Diacylglycerol (DAG) is a versatile lipid whose 1,2-sn-stereoisomer serves both as second messenger in signal transduction pathways that control vital cellular processes, and as metabolic precursor for downstream signaling lipids such as phosphatidic acid. Effector proteins translocate to available DAG pools in the membranes by using conserved homology 1 (C1) domains as DAG-sensing modules. PKCs define a central DAG-sensing node in intracellular phosphoinositide signaling pathways that regulate cell growth, differentiation, apoptosis, and motility. Herein, we report the high-resolution crystal structures of a C1 domain (C1B from PKCδ) complexed to DAG and to each of four potent PKC agonists that produce different biological readouts and that command intense therapeutic interest.

We crystallized apo C1Bδ under conditions similar to those used for the C1Bδ-DAG complex (but without detergent) for a direct comparison. We found the structure to be identical to the previously reported apo structure (1PTQ17) with a backbone r.m.s.d. of 0.4 Å. The apo structure superimposes well onto the structures of DAG-complexed C1Bδ, with the notable exception of the Trp252 sidechain. In the DAG complex, this sidechain is oriented towards the DAG tethered to the membrane-binding region, whereas in the apo C1Bδ it is oriented away from that region.

> MPHRFKVYNYMSPTFCDHCGSLLWGLVKQGLKCEDCGMNVHHKCREKVANLCG> MMTNLETRLSGADPVFARELHAQLVQALGDVKRRLLRGGTQ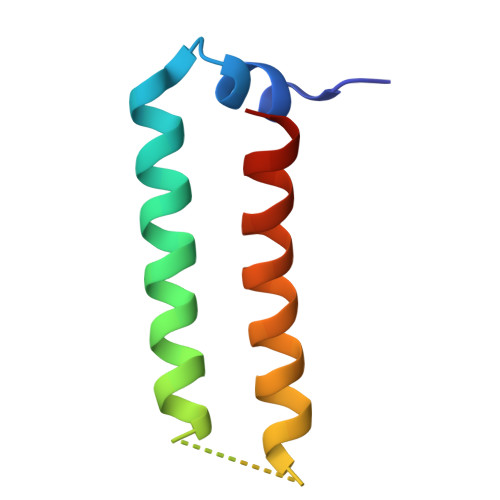QQYQQWQQEADAIEAGLNIIEKIKGE> MVEEVSNKQIIFKDYINGFPKESDMILKTSTIKLKVPEGCNDAVLVKNLYLSCDPYMRSRMSKLDDNYVPIFIPGSPITGDGVAKVLDSSHPDFKRGDLIRGITGWEEYTLIQSAEFITKIQHTDLPLSYHIGILGMPGLTAYAGFYEISS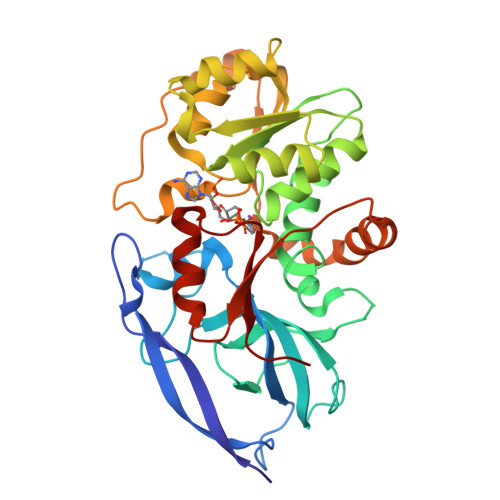PKEGETVFVSAASGAVGQLVGQFAKLSGCYVVGSAGTKDKVDMLKNKFGFDDAFNYKEEHDLDAALKRYFPEGIDIYFDNVGGKMLDAVLPNMKTKGRIATCGMISQYNLDEAEGVRNLFCIMTKQIRMQGYLVYYYRHLYPKLFDLVVPLLRQGKINYVEDVAEGLESAPAALIGLFSGRNVGKQVVRVATE> TKPVHLWTKPDVADWLESLNLGEHKEAFMDNEIDGSHLPNLQKEDLIDLGVTRVGHRMNIERALKQLL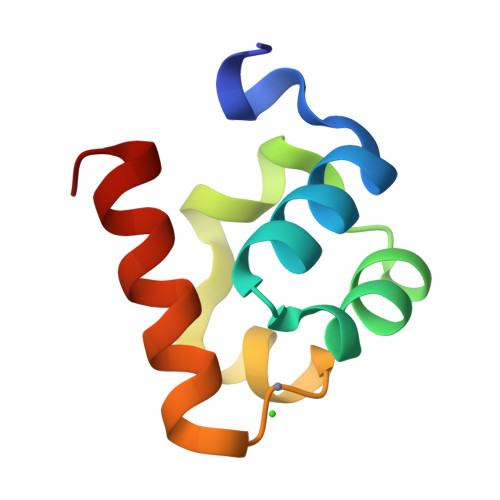DR> MGSSHHHHHHSQSLQEEAQGKTKKLKKVWTMLMAAKSE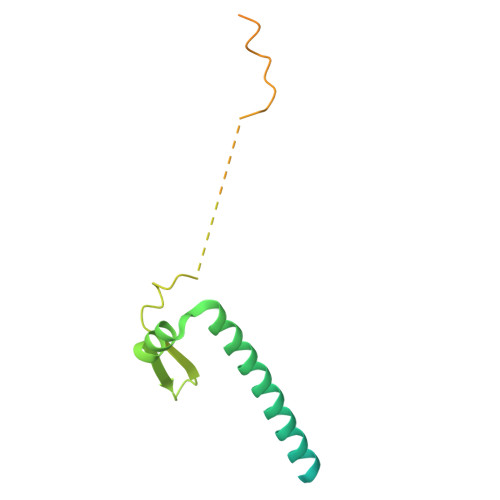MADLQQEHQREIEGLLENIRQLSRELRLQMLIIDNFIPQDYQEMIENYVHWNEDIGEWQLKCVAYTGNNMRKQTPVPDKKERDPFEVDLSHVYLAYTEESLRQSLMKLERPRTSKGKARPKMGRRKRSAKPETVIDSLLQ>MSISWTRNFFERFCVEEYNIDTIKQSSFLSADLLPSLGARINQSTKLRKHIISPFNPRYRAWEMWLVLLVIYSAWICPFQFAFITYKKDAIFIIDNIVNGFFAIDIILTFFVAYLDSHSYLLVDSPKKIAIRYLSTWFAFDVCSTAPFQPLSLLFNYNGSELGFRILSMLRLWRLRRVSSLFARLEKDIRFNYFWIRCTKLISVTLFAIHCAGCFNYLIADRYPNPRKTWIGAVYPNFKEASLWNRYVTALYWSITTLTTTGYGDFHAENPREMLFDIFFMMFNLGLTAYLIGNMTNLVVHWTSRTRTFRDSVRAASEFASRNQLPHDIQDQMLSHICLKFKTEGLKQQETLNNLPKAIRSSIANYLFFPIVHNIYLFQGVSRNFLFQLVSDIDAEYFPPKEDIILQNEAPTDLYILVSGAVDFTVYVDGHDQFQGKAVIGETFGEVGVLYYRPQPFTVRTTELSQILRISRTSLMSAMHAHADDGRVIMNNLFMKLRGQQSIAIDDSNTSGHENRDFKSMGWEEWRDSRKDGYGLDVTNPTSDTALMDAIHKEDTEMVKKILKEQKIERAKVERSSSETAGRSYANDSSKKDPYCSSSNQIIKPCKREEKRVTIHMMSESKNGKLILLPSSIEELLRLASEKFGGCNFTKITNADNAEIDDLDVIWDGDH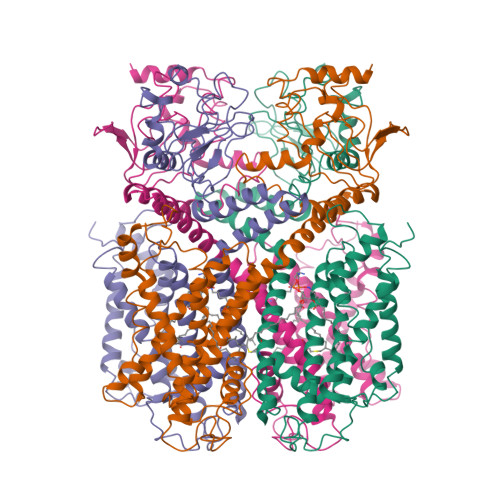LYFSSN[4x]>MDVFAKHAVSLESPAVRHYEITPSDSTDLARRPRALRVQTGGTLVLRDETGITVTYTVFAGEILPVRPVRVLATGTTATAVGWE[11x];>MPEGADPVAEVKTALAGFLKEVKGFQDDVKTRLQQQEERVTMLQTKTYAGRHALAAAATEEAPHQKAFAAYLRTGDDDGLRGLSLEGKALNSAVAAEGGYLVDPQTSETIRGVLRSTASLRQIASVVNVEATSFDVLVDKTDMGSGWASETAALSETATPQIDRITIPLHELAAMPKASQRLLDDSAFDIETWLANRIADKFARAEAAAFISGDGVDKPTGFLTKTKVANGAWAWGSLGYVATGAAGDFAAVNASDAVVDLVYALGAEYRANASFVMNSKTAGAVRKMKDADGRFLWADSLAAGEPARLMGYPVLIAEDMPDIAANAYAIAFGDFGNGYTIAERPDLRVLRDPFSAKPHVLFYASKRVGGDVSDFAAIKLLKFAAS[29x];>[2x]MIALGLGLGLAANGGPALRRYAVNGVAPVAVLDFERHFLSHPLALTRATSATYADALRAVQTAPADTPRYDYSTGKRALLLEASATNLLPNSAQFEAASWGKTRASVLANAALAPNGTMTADKLVEDTSNNSHFVARTGTQIAAGTSVTASIFVKAAERRWFALVTADSANAFRTTYFDLQTGTLGVVSQGAAGHVAQIVAAGNGWYRCSVTQTQAASGNFNFYPSVASANGATSYPGDGASGLYLWGAQLEAGAAVSSVIPTEAAAVTRAADLASVAVAAGSYDLRRVDAAGTA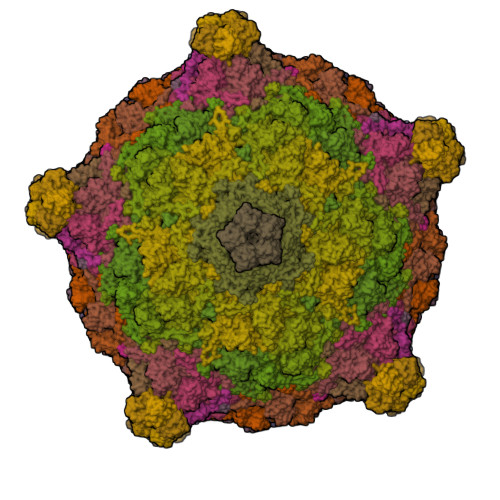VTKGVAHPGGALTIGAGSLYLLSLFPAGAL> EKSVVFKAEGEHFTDQKGNTIVGSGSGGTTKYFRIPAMCTTSKGTIVVFADARHNTASDQSFIDTAAARSTDGGKTWNKKIAIYNDRVNSKLSRVMDPTCIVANIQGRETILVMVGKWNNNDKTWGAYRDKAPDTDWDLVLYKSTDDGVTFSKVETNIHDIVTKNGTISAMLGGVGSGLQLNDGKLVFPVQMVRTKNITTVLNTSFIYSTDGITWSLPS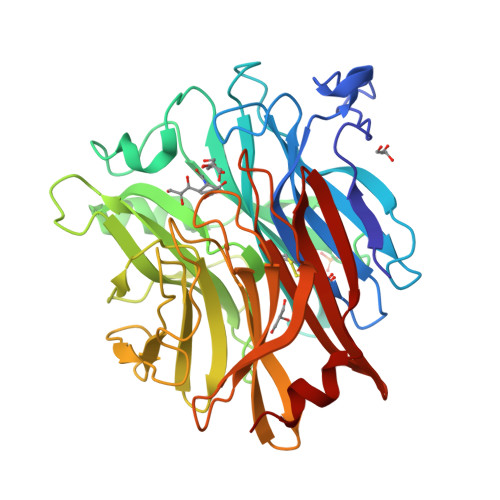GYCEGFGSENNIIEFNASLVNNIRNSGLRRSFETKDFGKTWTEFPPMDKKVDNRNHGVQGSTITIPSGNKLVAAHSSAQNKNNDYTRSDISLYAHNLYSGEVKLIDDFYPKVGNASGAGYSCLSYRKNVDKETLYVVYEANGSIEFQDLSRHLPVIKSYN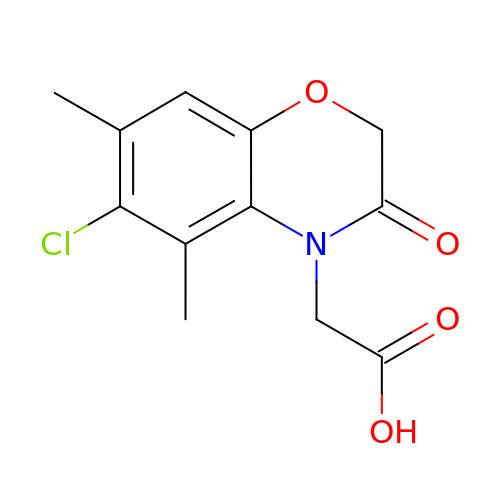2-(6-chloranyl-5,7-dimethyl-3-oxidanylidene-1,4-benzoxazin-4-yl)ethanoic acid | C12 H12 Cl N O4 | SUZXIGFIHWADFB-UHFFFAOYSA-N> GSDVAIVKEGWLHKRGEYIKTWRPRYFLLKNDGTFIGYKERPQDVDQREAPLNNFSVAQCQLMKTERPRPNTFIIRCLQWTTVIERTFHVETPEEREEWTTAIQTVADGLKKQAAAEMDFRSGSPSDNSGAEEMEVSLAKPKHRVTMNEFEYLKLLGKGTFGKVILVKEKATGRYYAMKILKKEVIVAKDEVAHTLTENRVLQNSRHPFLTALKYSFQTHDRLCFVMEYANGGELFFHLSRERVFSEDRARFYGAEIVSALDYLHSEKNVVYRDLKLENLMLDKDGHIKITDFGLCKEGIKDGATMKTFCGTPEYLAPEVLEDNDYGRAVDWWGLGVVMYEMMCGRLPFYNQDHEKLFELILMEEIRFPRTLGPEAKSLLSGLLKKDPKQRLGGGSEDAKEIMQHRFFAGIVWQHVYEKKLSPPFKPQVTSETDTRYFDEEFTAQM

The protein kinase Akt is a central signaling molecule within the PI3K/Akt/mTOR-pathway, and dysregulation and malfunction of this pathway is a major cause of human diseases such as cancer and diabetes. For the protein kinase Akt, three isoforms are encoded in the human genome sharing a high overall sequence homology, particularly within the conserved kinase and the pleckstrin homology (PH) domains. Recently, we utilized a class of covalent-allosteric Akt inhibitors (CAAIs) to achieve isoform-selectivity. These types of ligands alkylate one of two cysteine residues within an interdomain pocket between the regulatory PH and the catalytic kinase domain, leading to an irreversible stabilization of the inactive conformation bearing a structurally blocked ATP-binding site.

For a greater understanding of the binding mode of the synthesized ligands, we co-crystallized two Akt1-selective pyridine derivatives with full-length Akt1. The complex structures depict a similar binding mode and show that both ligands stabilize the full-length protein in the autoinhibited conformation with the PH domain folded onto the kinase domain (PH-in conformation). Through this intramolecular contact between the N- and the C-lobe, the regulatory helix αC is displaced, shaping an allosteric binding pocket at the interface. The kinase is stabilized in a DFG-out conformation. Due to missing interactions with adenosine or an equivalent moiety, the hinge region is slightly shifted. The relatively small biarylic part of the molecule is stabilized by π–π-stacking with Trp80 and Tyr272. Additional hydrophobic interactions can be observed between the phenyl ring in the 3-position and Leu210, Leu264, and Ile290. On the other hand, the complex with CAAI 3 highlighted a more flexible residue at the benzylic position of the pyridine core, which is close to Lys268. In both structures, the data suggested that the covalent inhibitors can label Cys310 and Cys296. Further structural proof was provided through co-crystallization of Akt1 with potent CAAIs 3 and 6, which revealed covalent bond formation to the addressed cysteine residues.>[4x]MRGSHHHHHHGSAKITTVIDIGSNSVRLAVFKKTSQFGF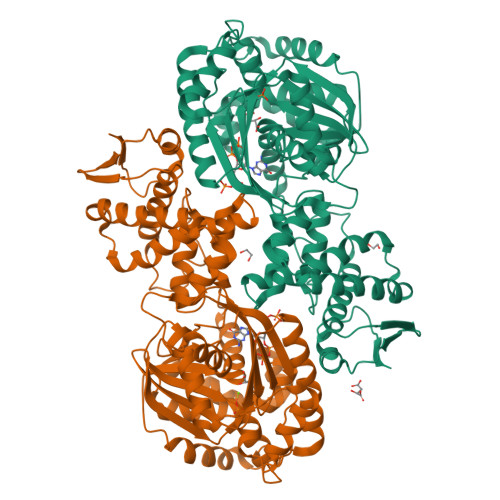YLLFETKSKVRISEGCYAFNGILQEIPMQRAVKALSEFKEIALKYKSKKILCVATSAVRDAPNRLEFVARVKKACGLQIKIIDGQKEALYGGIACANLLHKNSGITIDIGGGSTACALIEKGKIKDLISLDVGTIRIKEMFLDKDLDVKLAKAFIQKEVSKLPFKHKNAFGVGGTIRALSKVLMKRFDYPIDSLHGYEIDAHKNLAFIEKIVMLKEDQLRLLGVNEERLDSIRSGALILSVVLEHLKTSLMITSGVGVREGVFLSDLLRNHYHKFPPNINPSLISLKDRFLPHEKHSQKVKKECVKLFEALSPLHKIDEKYLFHLKIAGELASMGKILSVYLAHKHSAYFILNALSYGFSHQDRAIICLLAQFSHKKIPKDNAIAHMSAMMPSLLTLQWLSFILSLAENLCLTDSHHLKYTLEKNKLVIHSNDALYLAKEMLPKLVKPIPLTIEFA>[2x]MGHHHHHHGGWGGSGGENLYFQGDILIVNAKDVDEMLKQVEILRRLGAKQIAVHSSDWRILQEALKKGGDILIVNGGGMTITFRGDDLEALLK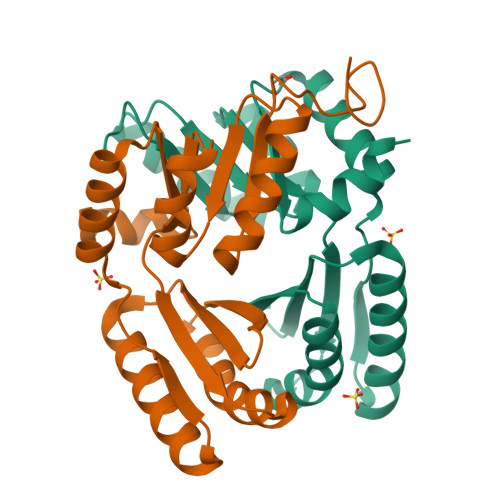AAIEMIKQALKFGATITLSLDGNDLNINITGVPEQVRKELAKEAERLAKEFGITVTRTGGGDVDEMLKQVEILRRLGAKQIAVESDDWRILQEALKKG Purine nucleoside phosphorylase (PNP, purine nucleoside orthophosphate ribosyl transferase, EC 2.4.2.1) has a crucial role in the purine salvage pathway. It catalyses the reversible phosphorolytic cleavage of the glycosidic bond of purine (2′-deoxy) nucleosides, generating the corresponding free base and (2′-deoxy) ribose 1-phosphate. E. coli PNP is an excellent molecular machine conducting efficient catalysis of purine nucleosides glycosidic bond cleavage. It is a homohexamer, built as a trimer of dimers, with all its subunits having the active site in the open conformation in the apo enzyme form. Monomers in each dimer mutually donate two amino acids (His4 and Arg43) to complete their active sites.

The crystal structure of complex WT-6(P/S)-6FA was obtained with a higher concentration of FA compared to structure WT-6(P/S)-2FA, and this resulted in filling all the active sites, including those in the open conformation. Difference electron density for omitted FA is best in the closed active site A, then in the open active site B, and finally somewhat poorer in the open active site D, which forms an open-closed dimer with site A. This is backed up by the values of occupancies of FA molecules, which in these three active sites are given as A:B:D = 0.8:0.5:0.4. This suggests that in the wild-type enzyme the active site B from the open-open B-B’ dimer exhibits a slightly higher affinity towards FA than the active site D that belongs to the closed-open A-D dimer. It turned out that the conformation of both proteins with all the active sites occupied by both ligands was the same, with a closed conformation in one of three active sites. Both ligands are in the same orientation in the active sites of WT and DM, and the conformation of crucial amino acids is very similar.

>ATPHINAEMGDFADVVLMPGDPLRAKYIAETFLEDAREVNNVRGMLGFTGTYKGRKISVMGHGMGIPSCSIYTKELITDFGVKKIIRVASCGAVLPHVKLRDVVIGMGACTDSKVNRIRFKDHDFAAIADFDMVRNAVDAAKALGIDARVGNLFSADLFYSPDGEMFDVMEKYGILGVEMEAAGIYGVAAEFGAKALTICTVSDHIRTHEQTTAAERQTTFNDMIKIALESVLLGDK[3x]In the barley β-d-glucan glucohydrolase, a glycoside hydrolase family 3 (GH3) enzyme, the Trp286/Trp434 clamp ensures β-d-glucosides binding, which is fundamental for substrate hydrolysis during plant growth and development. HvExoI folds into a two-domain structure consisting of an (α/β)8 barrel (domain 1) and an (α/β)6 sandwich (domain 2) with a 13 Å-deep active site pocket embracing the subsites −1 and +1, positioned at the interface between the two domains. HvExoI catalyses the hydrolytic removal of nonreducing glucose (Glc) moiety from a broad spectrum of poly- and oligomeric β-d-glucosides. The crucial role of substrate binding in HvExoI implies a pair of the aromatic Trp286 and Trp434 residues that form a clamp at the +1 subsite, which is positioned next to a pocket-shaped site at the −1 subsite, housing the Asp285 and Glu491 catalysts.

Of the tested mutants, W434H was the only mutant that exhibited broad substrate specificity similar to WT, contrary to W286F and W286Y, and W434F, W434Y, W286F/W434F, and W286F/W434A that lacked activities of at least with one carbohydrate substrate. The G2SG-OMe thio-analogue bound weakly to native and WT recombinant HvExoI with the respective Ki of 2 ×10−3 M and 4 ×10−3 M, reflecting its ability to attach at the +1 and +2 subsites instead of the −1 and +1 subsites, which was most likely due to the rigidity of this thio-ligand. On the other hand, in W286F the electron density map of G2SG-OMe was defined at the −1 and +1 subsites, where this thio-ligand formed H-bonds with Asp95, Lys206, His207, Arg158, Tyr253, Asp285, Arg291, and Glu491, and stacking interactions with W286F and Trp434, whereas G2SG-OMe did not bind to W286A and W286Y. The dispositions of G2SG-OMe at the −1 and +1 subsites in the W434A, W434F, W434H, and W434Y mutants revealed similar structural features of the ligand binding to those seen in W286F. As expected, the (1,3)- and (1,4)-linked thio-inhibitors were less potent with tested mutants, while the most effective thio-inhibitor was G6SG-OMe, except that it did not bind to W434A, and compared to WT, it showed 8- and 6-fold higher Ki constant values with W434H and W434F, respectively. These data pointed out that the replacements of Trp434 with Ala, His, or Phe residues in the +1 subsite, disturbed the optimal binding of thio-analogues, due to the removal or weakening stacking interactions crucial for the correct positioning of inhibitors in the active site. While Glc remained highly restrained in the −1 subsite in WT and W434H, it was mobile in W434A, hinting that the overall flexibility of the catalytic site was little affected in W434H, but strongly affected in W434A. GPathFinder simulations with W434H (Glc at the −1 subsite and laminaripentaose in the +1 and +2 subsites and bulk solvent), revealed that the Glc egress path was identical to that of WT (path 1).

> HHAADYVLYKDATKPVEDRVADLLGRMTLAEKIGQMTQIERLVATPDVLRDNFIGSLLSGGGSVPRKGATAKEWQDMVDGFQKACMSTRLGIPMIYGIDAVHGQNNVYGATIFPHNVGLGATRDPYLVKRIGEATALEVRATGIQYAFAPCIAVCRDPRWGRCYESYSEDRRIVQSMTELIPGLQGDVPKDFTSGMPFVAGKNKVAACAKHFVGDGGTVDGINENNTIINREGLMNIHMPAYKNAMDKGVSTVMISYSSWNGVKMHANQDLVTGYLKDTLKFKGFVISDWEGIDRITTPAGSDYSYSVKASILAGLDMIMVPNKYQQFISILTGHVNGGVIPMSRIDDAVTRILRVKFTMGLFENPYADPAMAEQLGKQEHRDLAREAARKSLVLLKNGKTSTDAPLLPLPKKAPKILVAGSHADNLGYQCGGWTIEHQGDTGRTTVGTTILEAVKAAVDPSTVVVFAENPDAEFVKSGGFSYAIVAVGEHPYTETKGDNLNLTIPEPGLSTVQAVCGGVRCATVLISGRPVVVQPLLAASDALVAAWLPGSEGQGVTDALFGDFGFTGRLPRTWFKSVDQLPMNVGDAHYDPLFRLGYGLTTNATKKY> SHDEPSESSEPCCDSC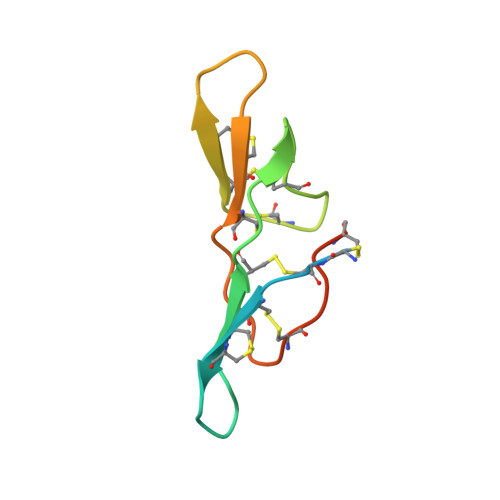DCTKSKPPQCHCANIRLNSCHSACKSCICTRSMPGKCRCLDTDDFCYKPCESMDKD The hypothetical protein Cyc15 was found to catalyse an intramolecular cycloaddition to generate a novel spirotetronate. Cyc15 shares 28 % sequence identity with AbyU and was identified in the draft genome of Streptomyces sp. NL15‐2 K as a hypothetical protein. The overall fold of Cyc15 is analogous to those reported for other spirotetronate cyclases, possessing an eight‐stranded antiparallel β‐barrel fold with (+1) 8 topology. Mechanistic studies indicate that these enzymes accelerate [4+2] cycloadditions via an asynchronous concerted mechanism, consistent with a formal Diels‐Alder reaction.

The structure reveals an asymmetric unit comprising two molecules of Cyc15 (Chain A and Chain B), which form a homodimer. Chain A comprises residues 9–148 of the full‐length polypeptide, with Chain B comprising residues 9–145. The AlphaFold search model aligns well with our experimentally determined crystal structure with a Cα RMSD of 0.47 Å. The Cyc15 dimer interface is populated predominantly by hydrophobic residues, along with a pair of equivalently positioned cysteines (Cys59; one contributed by each monomer) which sit 5 Å apart. Each Cyc15 monomer houses a large, solvent exposed active site cavity, which is sealed at one end by a salt bridge formed between the residues Glu17 and Arg122. Access to this site is regulated via a flexible loop, formed by the β1‐β2 linker (residues Asn25‐Met36), which caps the opposing end of the barrel. In our Cyc15 crystal structure electron density is only observed for the capping loop of Chain A, which is packed tightly against a symmetry partner. As a consequence of this arrangement, the side chain of Glu132 from each copy of Chain A extends into the entrance of the central cavity of a symmetry partner, forcing the recipients capping loop into an ‘open’ conformation. The Cyc15 active site is populated by a combination of hydrophobic and aromatic amino acids consistent with the required local environment for promotion of the [4+2] cycloaddition. Docking studies indicate a mode of substrate binding consistent with the formation of the diastereomer 3, providing a structural explanation for the observed stereochemical output of the Cyc15 catalysed reaction.

>[2x]MGDTTTANDVVTVELVEKVTKKDLNESGSIEGFGPGMMATYWCDVFDTEGKHIGTTVGCMDILYADPESGHLVEHVAEQIRLPDGTIMAWGTMNRSDVLAQKWITYRCQGTSGRYAGLVGTRTWRIQSLEDESYPIVAKMELRGALEHHHHHH>MVLLHKSTHIFPTDFASVSRAFFNRYPNPYSPHVLSIDTISRNVDQEGNLRTTRLLKKSGKLPTWVKPFLRGITETWIIEVSVVNPANSTMKTYTRNLDHTGIMKVEEYTTYQFDSATSSTIADSRVKFSSGFNMGIKSKVEDWSRTKFDENVKKSRMGMAFVIQKLEEA[2x];>SASFAPECTDLKTKYDSCFNEWYSEKFLKGKSVENECSKQWYAYTTCVNAALVKQGIKP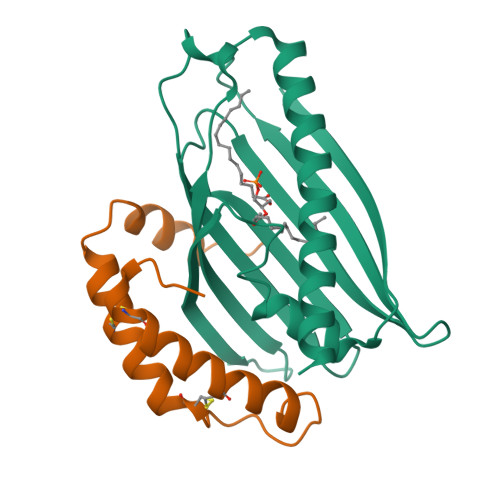ALDEAREEAPF[2x]CE2 enzymes are acetyl esterases (that are generally not appended to other catalytic modules), which are reported to be active on synthetic aryl-esters and acetylated xylan. Here we report the biochemical properties and crystal structure of several CE2 members, both single-module CE2 enzymes and CtCE2, a component of CtCel5C-CE2. All three 3D structures reveal a bi-domain enzyme in which an N-terminal β-sheet “jelly roll” domain (around 130 residues) is linked to a C-terminal domain of approximately 220 residues. The C-terminal domains possess an atypical α/β-hydrolase (SGNH-hydrolase) fold, consisting of repeating β-α-β motifs that form a curved central five-stranded parallel β-sheet, in the strand order β2, β1, β3, β4, and β5 with strand β2 interrupted by loop insertion.

The bacterium Clostridium thermocellum contains a single CE2 member, designated CtCE2, which is linked to the cellulase, CtCel5C, within the modular protein designated CtCel5C-CE2. In this enzyme the oxyanion hole, similar to CjCE2A, comprise the N of Ser-612 and Gly-658 and the Nδ2 of Asn-705 with formate again mimicking the tetrahedral transition state. The structure of the α/β-hydrolase domain of CtCE2 revealed a deep cleft. The structure of both wild-type CtCE2 and the S612A mutant were determined in the presence of cellohexaose and clear electron density for five β-1,4-linked d-glucose molecules was observed in the cleft, consistent with the affinities revealed by ITC. The interaction of the oligosaccharide with CtCE2 is dominated by planar hydrophobic contacts between the pyranose rings of Glc-1 with Trp-746, Glc-2 and Trp-790, and Glc-4 and Tyr-665. In CtCE2, interaction of cellohexaose with the hydrophobic platform is augmented by several polar contacts. Notably, the O6 of Glc-4 makes a hydrogen bond with Oγ of Ser-612 (in one of its two conformations) in the wild-type esterase and Nɛ2 of His-791 in the S612A mutant, while O6 of Glc-2 interacts with Oɛ1 of Gln-780. As was revealed in the 3-D complex structure and discussed in more detail below, cellooligosaccharide binding, with a stoichiometry of 1, occurs across the esterase active centre with both the Ser and His of the dyad influencing ligand recognition. The importance of all three hydrophobic interactions in the binding of CtCE2 to cellulose was demonstrated by the observation that the mutants W746A, W790A, and Y665A displayed no, or extremely weak, affinity for cellohexaose or β-glucan.

> MASPDEDNPGILYNGRFDFSDPNGPKCAWSGSNVELNFYGTEASVTIKSGGENWFQAIVDGNPLPPFSVNATTSTVKLVSGLAEGAHHLVLWKRTEASLGEVQFLGFDFGSGKLLAAPKPLERKIEFIGDSITCAYGNEGTSKEQSFTPKNENSYMSYAAITARNLNASANMIAWSGIGLTMNYGGAPGPLIMDRYPYTLPYSGVRWDFSKYVPQVVVINLGTNDFSTSFADKTKFVTAYKNLISEVRRNYPDAHIFCCVGPMLWGTGLDLCRSYVTEVVNDCNRSGDLKVYFVEFPQQDGSTGYGEDWHPSIATHQLMAERLTAEIKNKLGWLEHHHHHH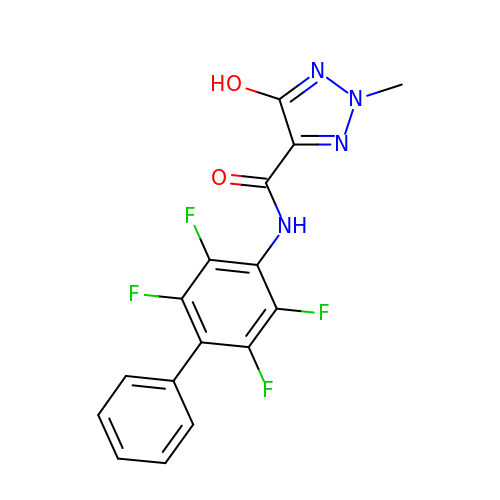2-methyl-5-oxidanyl-~{N}-[2,3,5,6-tetrakis(fluoranyl)-4-phenyl-phenyl]-1,2,3-triazole-4-carboxamide | C16 H10 F4 N4 O2 | NRGHNOMCGATBLG-UHFFFAOYSA-N> MRLLTALFAYFIVALILAFSVSAKSMSERRAVYIGALFPMSGGWPGGQACQPAVEMALEDVNSRRDILPDYELKLIHHDSKCDPGQATKYLYELLYNDPIKIILMPGCSSVSTLVAEAARMWNLIVLSYGSSSPALSNRQRFPTFFRTHPSATLHNPTRVKLFEKWGWKKIATIQQTTEVFTSTLDDLEERVKEAGIEITFRQSFFSDPAVPVKNLKRQDARIIVGLFYETEARKVFCEVYKERLFGKKYVWFLIGWYADNWFKIYDPSINCTVDEMTEAVEGHITTEIVMLNPANTRSISNMTSQEFVEKLTKRLKRHPEETGGFQEAPLAYDAIWALALALNKTSGGGGRSGVRLEDFNYNNQTITDQIYRAMNSSSFEGVSGHVVFDASGSRMAWTLIEQLQGGSYKKIGYYDSTKDDLSWSKTDKWIGGSPPADQTLVIKTFRFLSQKLFISVSVLSSLGIVLAVVCLSFNIYNSHVRYIQNSQPNLNNLTAVGCSLALAAVFPLGLDGYHIGRNQFPFVCQARLWLLGLGFSLGYGSMFTKIWWVHTVFTKKEEKKEWRKTLEPWKLYATVGLLVGMDVLTLAIWQIVDPLHRTIETFAKEEPKEDIDVSILPQLEHCSSRK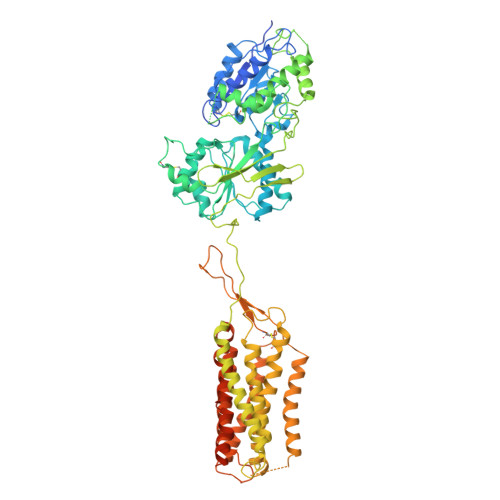MNTWLGIFYGYKGLLLLLGIFLAYETKSVSTEKINDHRAVGMAIYNVAVLCLITAPVTMILSSQQDAAFAFASLAIVFSSYITLVVLFVPKMRRLITRGEWQSEAQDTMKTGSSTNNNEEEKSRLLEKENRELEKSGRLEVLFQ ETHYL 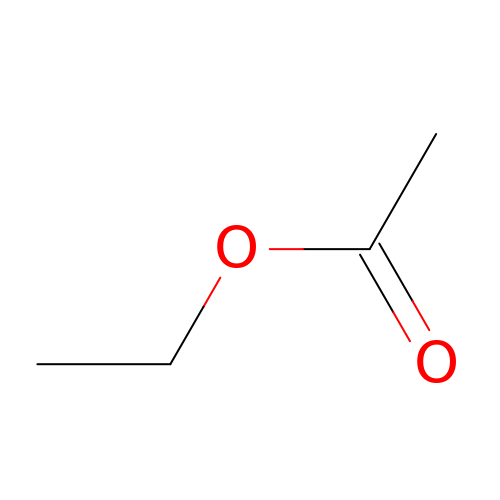ACETATE | C4 H8 O2 | XEKOWRVHYACXOJ-UHFFFAOYSA-N> GSNVNKIYIENHDLMSKVPVIEASKESTRDDWAALTVVADLDDIEGQELVYYALRFRKSNDGVRLDIVHNPKDTSRSPSVLAQRLKSREDKLLDFTRFLDLETALETGEFEPDVAYDASLANFLASSNMKAGDNFVILNGRVLGPITSADDFKKEDFEVFLQA

UGGT acts as the gatekeeper in this system because this enzyme is capable of sensing the folding states of glycoproteins as potential substrates. UGGT only transfers monoglucose residues to incompletely folded glycoproteins. UGGT is a large enzyme, comprising approximately 1500 amino acid residues, which has been putatively divided into two regions: an N-terminal folding-sensor region, which accounts for approximately 80% of the enzyme and is not homologous with any known structures, and a C-terminal catalytic domain, which accounts for the remaining 20% of the enzyme and belongs to the glycosyltransferase 8 family. On the other hand, the folding-sensor region of UGGT was found to harbour three tandem Trx-like domains: Trx1 (residues 168–379), Trx2 (residues 467–624) and Trx3 (residues 671–831).

On the other hand, Form 2 of the Trx3 domain of UGGT cocrystallized with a detergent ANAPOE C12E8 belonged to space group C2221 and diffracted up to 1.70-Å resolution. In the crystal structure, one molecule was contained per asymmetric unit. The final model of Form 2 had an Rwork of 20.1% and Rfree of 24.6%. The C-terminal α6 helix, which is followed by a putatively flexible linker region in UGGT, was completely disordered in the crystal structure of Form 2, suggesting the instability of this helix (left). Because of the absence of the α6 helix, an extensive hydrophobic patch was exposed on the surface of the Trx3 domain (centre). The detergent ANAPOE C12E8 was accommodated on this exposed hydrophobic patch. Most of these hydrophobic residues were involved in the interaction with the detergent in Form 2. Thus, the C-terminal α6 helix and detergent molecule occupy the common hydrophobic surface of the Trx3 domain. Although we cannot exclude the possibility that the hydrophobic patch of the Trx3 domain is covered by other domain(s) in intact UGGT, the flexible properties of the C-terminal helix of Trx3 may contribute to regulatory mechanisms underlying the folding-sensing function of this domain. Thus, our crystallographic study provides an atomic view of the potential substrate-binding site of UGGT.Recently, the bacterial strain Ideonella sakaiensis 201-F6 was discovered and shown to grow on low-crystallinity PET films. Two α/β-hydrolase fold enzymes (α/β-hydrolases), PETase and MHETase, work together to degrade PET in two steps via MHET, yielding TPA and ethylene glycol—the building blocks required for a new round of PET synthesis. We have determined crystal structures of recombinantly expressed and purified I. sakaiensis MHETase in its ligand-free form (2.05 Å resolution), MHETase bound to a nonhydrolyzable mono-(2-hydroxyethyl) terephthalamide (MHETA, 2.1 Å resolution) or to benzoic acid (BA, 2.2 Å resolution) as well as ligand-free PETase (2.0 Å resolution) (2a−f). PETase and MHETase only share the α/β-hydrolase fold (2.87 Å RMSD for 184 out of 262 residues aligned).

The overall domain architecture of the 65 kDa MHETase resembles that of feruloyl esterases, with a lid domain inserted between β-strand 7 and α-helix 15 of the α/β-hydrolase fold. As previously observed for feruloyl esterases, the presence of a structural calcium-binding site was confirmed by X-ray fluorescence spectroscopy for MHETase. Likewise, one of five disulfide bonds is flanking a catalytic triad (formed by S225, H528, D492) and the oxyanion hole comprising the backbone amide nitrogen atoms of G132 and E226. In the ligand-free structure of MHETase, several water molecules are maintained by a hydrogen bond network at the substrate-binding site. Despite their overall high similarity, a detailed comparison of MHETase structures in the absence and presence of the substrate reveals an induced-fit mechanism upon MHETA binding. In the ligand-free structure, F415 points away from the active site and thus opens it for substrate binding. While the α/β-hydrolase domain superimposes well with the closest structurally characterized feruloyl esterase homolog FaeB from A. oryzae (1.60 Å RMSD for 280 out of 342 residues aligned, 32.5% amino acid identity), the lid domain of MHETase contains several additional loops that markedly differ from FaeB (2.33 Å RMSD for 148 out of 215 residues aligned, 18.9% identity). The overall structures of MHETase and FaeB are structurally similar (2.04 Å RMSD for 421 out of 559 residues aligned) despite a relatively low number of amino acid identities (27.5%). When comparing MHETase with known tannase structures, e.g tannin acyl α/β-hydrolase from Lactobacillus plantarum (LptE), it is evident that only the overall fold of the α/β-hydrolase domain is similar (2.77 Å RMSD for 195 out of 282 residues aligned, 13.8% identity), while very large differences (5.24 Å RMSD) are observed for the lid domain. Contrasting consensus α/β-hydrolases, the bipartite architecture of MHETase parts catalysis from substrate recognition—a scenario where we envision the lid domain as a tunable platform to enhance catalytic properties (e.g. alleviating substrate release) or alter substrate specificity (as shown initially for the S416A, R411Q or F424N mutants reported here).

>MNHKVHHHHHHMGGGSTPLPLPQQQPPQQEPPPPPVPLASRAACEALKDGNGDMVWPNAATVVEVAAWRDAAPATASAAALPEHCEVSGAIAKRTGIDGYPYEIKFRLRMPAEWNGRFFMEGGSGTNGSLSAATGSIGGGQIASALSRNFATIATDGGHDNAVNDNPDALGTVAFGLDPQARLDMGYNSYDQVTQAGKAAVARFYGRAADKSYFIGCSEGGREGMMLSQRFPSHYDGIVAGAPGYQLPKAGISGAWTTQSLAPAAVGLDAQGVPLINKSFSDADLHLLSQAILGTCDALDGLADGIVDNYRACQAAFDPATAANPANGQALQCVGAKTADCLSPVQVTAIKRAMAGPVNSAGTPLYNRWAWDAGMSGLSGTTYNQGWRSWWLGSFNSSANNAQRVSGFSARSWLVDFATPPEPMPMTQVAARMMKFDFDIDPLKIWATSGQFTQSSMDWHGATSTDLAAFRDRGGKMILYHGMSDAAFSALDTADYYERLGAAMPGAAGFARLFLVPGMNHCSGGPGTDRFDMLTPLVAWVERGEAPDQISAWSGTPGYFGVAARTRPLCPYPQIARYKGSGDINTEANFACAAPP[10x]>[6x]MDLTNKNVIFVAALGGIGLDTSRELVKRNLKNFVILDRVENPTALAELKAINPKVNITFHTYDVTVPVAESKKLLKKIFDQLKTVDILINGAGILDDHQIERTIAINFTGLVNVTTAILDFWDKRKGGPGGIIANICSVTGFNAIHQVPVYSASKAAVVSFTNSLAKLAPITGVTAYSIN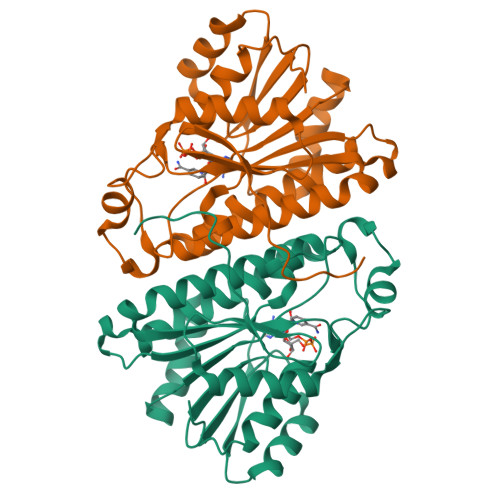PGITRTPLVHTFNSWLDVEPRVAELLLSHPTQTSEQCGQNFVKAIEANKNGAIWKLDLGTLEAIEWTKHWDSHI>TYTTRQIGAKNTLEYKVYIEKDGKPVSAFHDIPLYADKENNIFNMVVEIPRWTNAKLEITKEETLNPIIQDTKKGKLRFVRNCFPHHGYIHNYGAFPQTWEDPNVSHPETKAVGDNDPIDVLEIGETIAYTGQVKQVKALGIMALLDE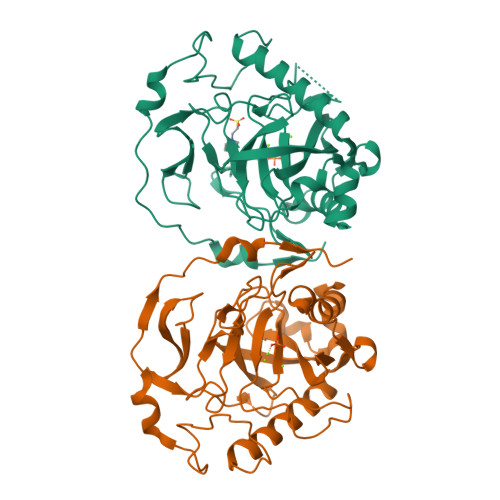GETDWKVIAIDINDPLAPKLNDIEDVEKYFPGLLRATNEWFRIYKIPDGKPENQFAFSGEAKNKKYALDIIKETHDSWKQLIAGKSSDSKGIDLTNVTLPDTPTYSKAASDAIPPASLKADAPIDKSIDKWFFISGSV[2x]> GSHMQEQDAGLDALSS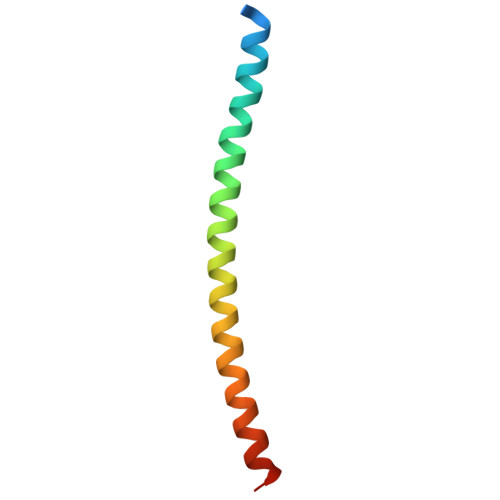IISRQKQMGQEIGNELDEQNEIIDDLANLVENTDEKLRTEARRVTLVDR>[2x]MDIAKWVEHARTCYSTQLDTKIKVIGVIGKDYPDHGKGDNINCYLRENVFPVAATEDETCTIRGHFSEDDQILFLVMNGVDDVANIRKCLKSNPKSNYFDAMAESECQQIRMLHFLFISCHFIIIFEQTSRIDLELMRFLKKVNSARIQLRKKINQRLVASDLRDVSFNNRILSSAESEGRMVVPRLLIAFQRNNIRPDVNPGKKLQRELYEKLEKNLDNQFSDILKLYDLIDCGASSLCQLNETIPVVHLLNPKIVKRDIIGEMFEILMADAENTKISGNAGTLPSNNSFVKFLEDNFRSEKNEISLENVIELMNCLQCVLDGDLEEKHEKTAIQTFIKRIQNDHMEEARRLYTNAQRPGERRGADRFKDSEKPVKIRSKEEHLMRFNEATHYIDSVVGVNSREALSQLQAQCNEMWQSDMRHHHHHH;> MKESVRFLTDFGEISDAISDLLTSSPNFNVISAIGPQGAGKSTLLSMLAGNNSRQMYREYVFRPVSREANEQSRHQTIQIDIYIVNHQIFLDCQPMYSFSIMEGLPKVRGGRFDDSTAMSDTLRLTAFLLYVSHTVLVVSETHYDKVIIDTLRVAEQIRPYLAIFRPKLAIDRKTNLVFIKTKASSIDLAPTVIREREELLRLSFQDSRWLKVSQEPFKTLIVLEEIRVRREHLFEEGDEPDEAASLNEFDEQIAELREELQKNREDFTVETAAMDEKKWLDMCREVIRDKTLHKTLKEYQRAMTDGVRTHFDNGFH;>MKESVRFLTDFGEISDAISDLLTSSPNFNVISAIGPQGAGKSTLLSMLAGNNSRQMYREYVFRPVSREANEQSRHQTIQIDIYIVNHQIFLDCQPMYSFSIMEGLPKVRGGRFDDSTAMSDTLRLTAFLLYVSHTVLVVSETHYDKVIIDTLRVAEQIRPYLAIFRPKLAIDRKTNLVFIKTKASSIDLAPTVIREREELLRLSFQDSRWLKVSQEPFKTLIVLEEIRVRREHLFEEGDEPDEAASLNEFDEQIAELREELQKNREDFTVETAAMDEKKWLDMCREVIRDKTLHKTLKEYQRAMT[2x];> MDIAKWVEHARTCYSTQLDTKIKVIGVIGKDYPDHGKGDNINCYLRENVFPVAATEDETCTIRGHFSEDDQILFLVMNGVDDVANIRKCLKSNPKSNYFDAMAESECQQIRMLHFLFISCHFIIIFEQTSRIDLELMRFLKKVNSARIQLRKKINQRLVASDLRDVSFNNRILSSAESEGRMVVPRLLIAFQRNNIRPDVNPGKKLQRELYEKLEKNLDNQFSDILKLYDLIDCGASSLCQLNETIPVVHLLNPKIVKRDIIGEMFEILMADAENTKISGNAGTLPSNNSFVKFLEDNFRSEKNEISLENVIELMNCLQCVLDGDLEEKHEKTAIQTFIKRIQNDHMEEARRLYTNAQRPGERRGADRFKDSEKPVKIRSKEEHLMRFNEATHYIDSVVGVNSREALSQLQAQCNEMWQ

The SMG1 kinase is an essential NMD factor in metazoans and is associated with two recently identified and yet poorly characterized proteins, SMG8 and SMG9. We found that SMG8–SMG9 is a G-domain heterodimer with architectural similarities to the dynamin-like family of GTPases such as Atlastin and GBP1. SMG8 and SMG9 interact with each other and inhibit the kinase activity of SMG1 in vitro. Nucleotide binding occurs at the G domain of SMG9 but not of SMG8.

Using bioinformatics analyses and proteolysis experiments, we identified regions C. elegans (C.e.) full-length SMG8 (873 residues) and SMG9 (385 residues) as sufficient to form a stable heterodimeric core complex (SMG8c, residues 1–423 and SMG9c, residues 59–375) and to yield diffracting crystals. After overcoming crystal lattice defects (detailed in Materials and Methods), we solved the structure and refined it at 2.5 Å resolution with Rfree of 26.0%. SMG8c and SMG9c contain a similar globular fold with characteristic architecture of G domains along with additional secondary structure elements. The major structural difference between SMG8c and SMG9c is the presence in the former of a helical bundle of three C-terminal helices (α7–α9) that forms a stalk-like protrusion reminiscent of the stalk domain found in GTPases of the dynamin family, such as Atlastin and GBP1 (Daumke and Praefcke 2016). The G domains of SMG8c and SMG9c face each other and interact with part of their convex surfaces. In particular, SMG8c helix α2A interacts with SMG9c helices α4 and α3 (patch 1) (in particular Val83SMG8, Ile86SMG8 with Leu258SMG9, Leu261SMG9). In addition, the stalk domain of SMG8c folds back on the convex surface of SMG9c (patch 2). Here, SMG8c stalk helices α2B and α7 interact with SMG9c helices α7 and α3 (e.g., Ile335SMG8 and Phe338SMG8 with Val212SMG9 and Tyr358SMG9). The SMG8–SMG9 heterodimer forms in the absence of nucleotides, with interactions conserved from worms to humans. Finally, the SMG8c–SMG9c heterodimer is formed irrespective of nucleotides, while proteins such as Atlastin or GBP1 dimerize in the presence of GTP analogs.An alternative to the classical Birch reduction is provided by dearomatizing benzoyl-coenzyme A (BzCoA) reductases (BCRs) from anaerobic bacteria. BCRs reduce their substrate to cyclohexa-1,5-diene-1-carbonyl-CoA (dienoyl-CoA), representing an ortho- rather than the para-dihydro addition of classical Birch reductions. Architecturally, the heterotetrameric enzyme complexes are composed of two functional dimers: the ATP-binding dimer coordinates a subunit-bridging [4Fe-4S] cluster and serves as an ATP-dependent electron activator, whereas the catalytic dimer is predicted to contain an FeS cluster in each subunit and the substrate binding site. In this study, we heterologously produced the active site components BzdNO from Aromatoleum sp. CIB and provide a first X-ray structural characterization of the catalytic dimer of a class I BCR with the BzCoA substrate and the dienoyl-CoA product in van der Waals contact with the catalytic FeS cluster.

BzCoA is embedded inside the active site channel of BzdO in an elongated fashion from the buried benzoyl head to the diphosphate of CoA at the channel entrance. After the diphosphate, CoA is kinked by ca. 90° and the 3’-phosphorylated adenosine tail is attached along the protein surface. The benzoyl ring of CoA is laterally displaced relative to the [4Fe-4S] cluster, such that the OH2/OH group points to on one side slightly above the benzoyl plane of the substrate. Trp46, Leu302, Leu383 and Tyr97 protruding from the N- and C-terminal α/β domains create a predominantly hydrophobic environment of the benzoyl ring. Access of bulk solvent to the active site is completely blocked. While C1, C2 and C6 of the benzoyl ring are not directly adjacent to protonable residues, C4 is 3.1 Å apart from the [4Fe-4S]-OH2/OH group and C3 is 3.6–4.0 Å from the [4Fe-4S]-OH2/OH group, Glu65-OE2 and Ser44-OG. The thioester oxygen of BzCoA is hydrogen-bonded with Tyr97, Tyr298 and Gln274 suitable for stabilizing negative charges by hydrogen-bond interactions. The four irons are coordinated to three cysteines (Cys95, Cys128 and Cys380) and a small non-proteinogenic ligand assigned as water (–OH2) or hydroxy (–OH) group indistinguishable at the current resolution. The structure of BzdNO with the bound BzCoA substrate was used as a starting model for quantum mechanics/molecular mechanics (QM/MM) calculations.

>[2x]MNAMANKYPTEQLKLWGKAKELREQYYMNYARAKEKGGIRWSGSAWALDAIPAGLGEDVYSLTGEPYAAAVAHDRKFAKECMDAAEAYGFARDLCSYMRIYWGGMHLNKYAFGGEFPKPDFVFQTQICCSHSKWYQHVAKEEKIPEFYLDVGVGPYRDMTDARLDYVANQLHDGIAFVEKASGRKFDDELFIKAVKNEMRSTSRWADICALNKVKPAPLDEKTMYSLYVLCTLSKSSQWCADFMDELYEEVKDRVARGIAAVPNEAIRLMTDTQPPWSFLKIFRYLETYGAVSIGSLYTFALEGIWEDKPDGSWGGRTLPWDKGIEINDRDTAVRLYADWNLSKPQWQHFYDPTIKSDMMLRIIKEWQVDGVMLHLNRGCEGLSVGIMENRLAIAKSGTPVMTFEGNMGDEREFDEVRTQARVDAFMEQLGVRRQAASAWSHPQFEK;>MSDGLFDQFKTWYEKRHDYARDWKVRTGGQVVATMCTYTPEELLIAAGMLPVRVLGAHEPQNVTEPHIFGMFCPFCRDSLAQGLLGRFDYAEGVTLTQSCIQYRQTFGSWRLHVPTVKWDYYVPMPNEVQSPHARKAHYEEVQAFRVFLQTLTGKEITDAMLSDALAVCDENRRLLRELYEYRKAADPKVTGVEALYASLTAQFIDKREHNEMLKKTLAALPNRKVERKTGARFMTIGSENDDIAFMGMVESVGATIVIDDQCSGSRYFWNASKPEGDVIKAIAERYCDRPACPTKDYPAHTRFDHVLGMAKEYNVEGAIFLQQKFCDPHEGDYPDLKRHLEENGIPTLFLEFDITNPIGPFRIRIEAFLETLSEEELF[2x]>[2x]GSHMPTAIESCMVKFELSSSKWHMTSPKPHCVNTTSDGKLKILQSGTYLIYG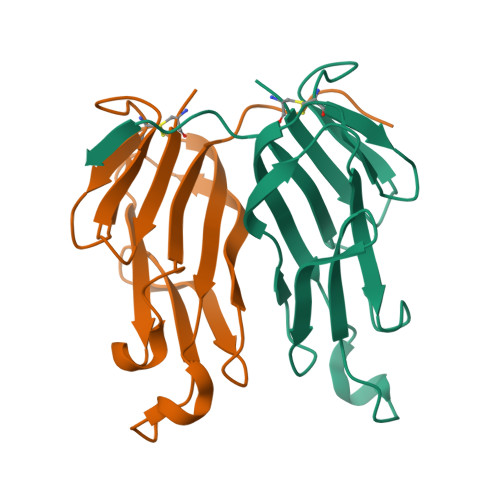QVIPVDKKYIKDNAPFVVQIYKKNDVLQTLMNDFQILPIGGVYELHAGDNIYLKFNSKDHIQKTNTYWGIILMPDLPFIS> MGSSHHHHHHSQDPKPRVLVLTGAGISAESGIRTFRAADGLWEEHRVEDVATPEGFDRDPELVQAFYNARRRQLQQPEIQPNAAHLALAKLQDALGDRFLLVTQNIDNLHERAGNTNVIHMHGELLKVRCSQSGQVLDWTGDVTPEDKCHCCQFPAPLRPHVVWFGEMPLGMDEIYMALSMADIFIAIGTSGHVYPAAGFVHEAKLHGAHTVELNLEPSQVGNEFAEKYY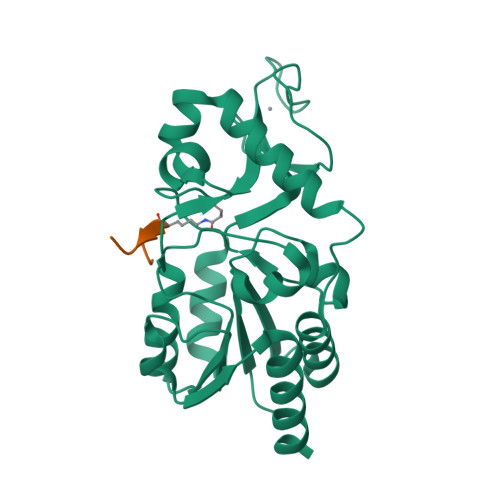GPASQVVPEFVEKLLKGLKAGSIA;> KGGAXRHRKIL> SEHTLAVSDSSFDQDVLKASGLVLVDFWAEWCGPCKMIGPALGEIGKEFAGKVTVAKVNIDDNPETPNAYQVRSIPTLMLVRDGKVIDKK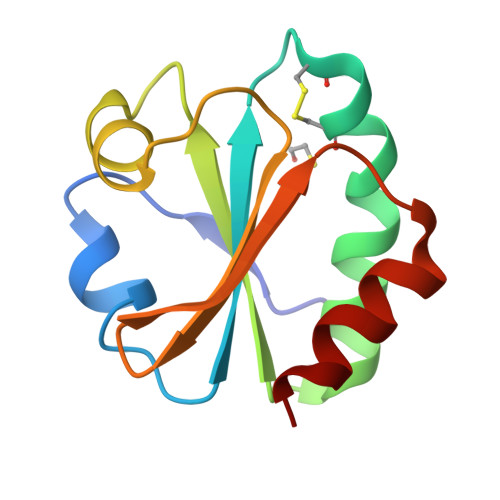VGALPKSQLKAWVESAQ>TTGERLIRVLQDQLKTLQRNYGRLQQDVLQF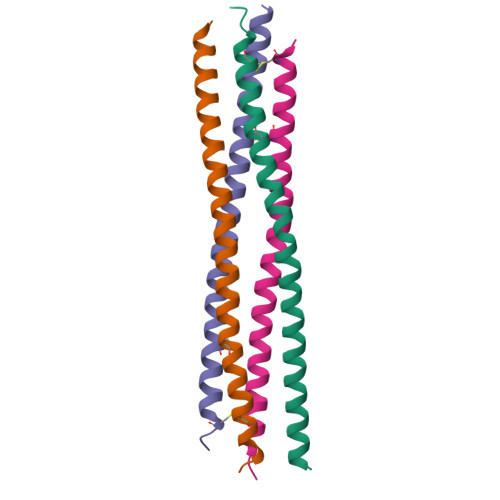QKNQTNLERKFSYDLSQCINQMKEVKEQCEERIEEV[4x]2-{[(4-iodophenyl)sulfonyl]amino}benzoic acid | C13 H10 I N O4 S | 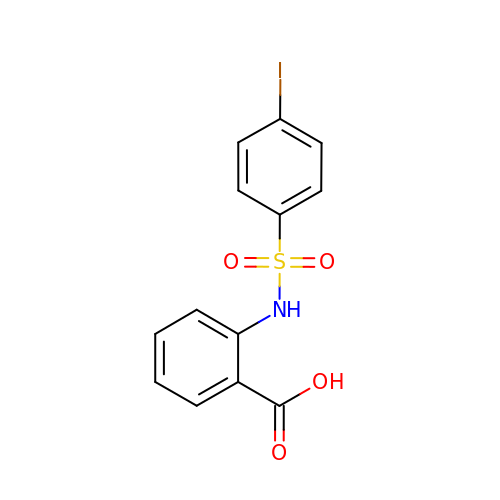PLJIQKJMJAHNRG-UHFFFAOYSA-N> MSGLRTVSASSGNGKSYDSIMKILLIGDSGVGKSCLLVRFVEDKFNPSFITTIGIDFKIKTVDINGKKVKL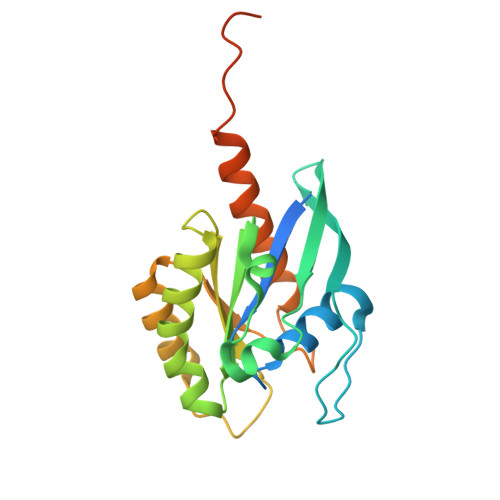QLWDTAGQERFRTITTAYYRGAMGIILVYDVTDERTFTNIKQWFKTVNEHANDEAQLLLVGNKSDMETRVVTADQGEALAKELGIPFIESSAKNDDNVNEIFFTLAKLIQEKIDSNKLVGVGNGKEGNISINSGSGNSSKSN> MESPSSEEEKPLAKMAFTLADRVTEEMLADKAALVVEVVEENYHDAPIVGIAVVNEHGRFFLRPETALADPQFVAWLGDETKKKSMFDSKRAAVALKWKGIELCGVSFDLLLAAYLLDPAQGVDDVAAAAKMKQYEAVRPDEAVYGKGAKRAVPDEPVLAEHLVRKAAAIWELERPFLDELRRNEQDRLLVELEQPLSSILAEMEFAGVKVDTKRLEQMGKELAEQLGTVEQRIYELAGQEFNINSPKQLGVILFEKLQLPVLKKTKTGYSTSADVLEKLAPYHEIVENILHYRQLGKLQSTYIEGLLKVVRPATKKVHTIFNQALTQTGRLSSTEPNLQNIPIRLEEGRKIRQAF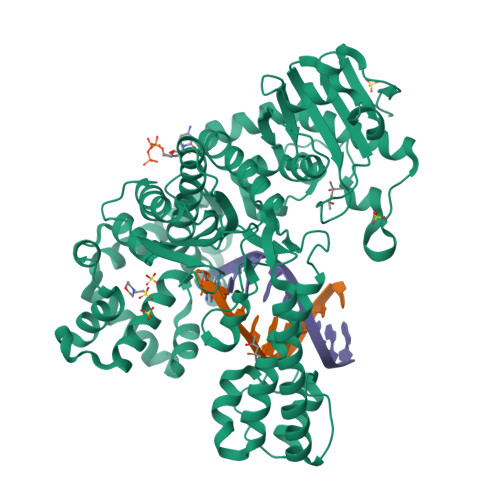VPSESDWLIFAADYSQIALRVLAHIAEDDNLMEAFRRDLDIHTKTAMDIFQVSEDEVTPNMRRQAKAVNFGIVYGISDYGLAQNLNISRKEAAEFIERYFESFPGVKRYMENIVQEAKQKGYVTTLLHRRRYLPDITSRNFNVRSFAERMAMNTPIQGSAADIIKKAMIDLNARLKEERLQAHLLLQVHDELILEAPKEEMERLCRLVPEVMEQAVTLRVPLKVDYHYGSTWYDAK>[2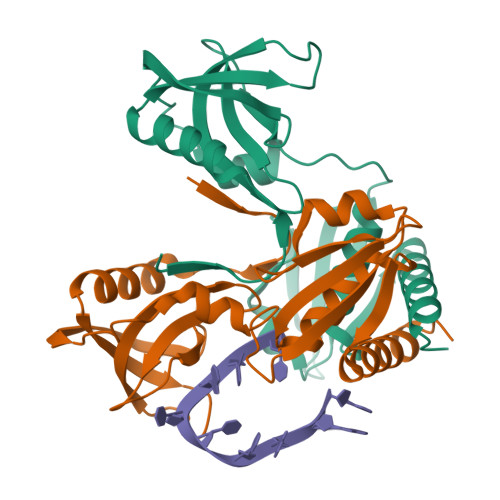x]GSHMETIAVHAGPRPYEDQAVLGAIRAAIKGLQALSFRYEGGSTPGRTREVTPLGVLFGRSNYLVALEGKGGKPRSWRLDRMSDLKVLDKPAPPPQDFSLQAFADESFGIYHDEIQDVVLRIHKSRAEDALRWRFHATQQVTPEADGSVLVTFRAGGMRELSWHLFTWGDAVEIVAPQVLKDMMVQELREAGRAHGAW N-[2-(benzoylamino)ethyl]-N-(biphenyl-4-ylsulfonyl)-D-valine | C26 H28 N2 O5 S | 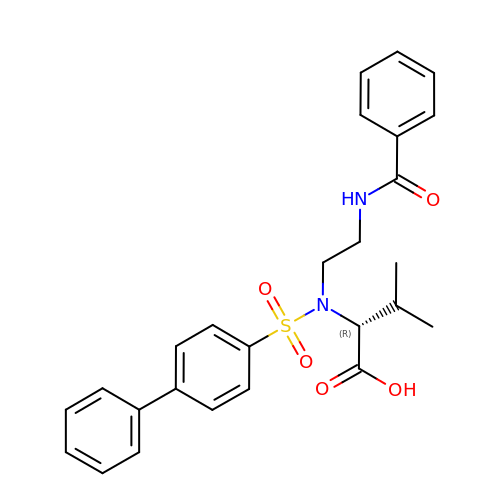BKYHPXRQAHYJBN-XMMPIXPASA-N>[2x]EFTQLSQSIAEFHTYQLGNGRCSSLLAQRI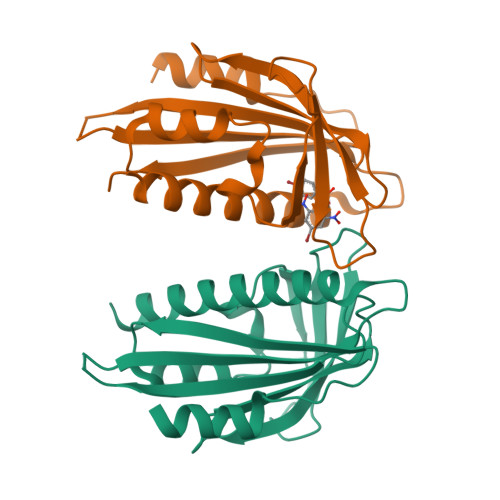HAPPETVWSVVRRFDRPQIYKHFIKSCNVSEDFEMRVGCTRDVNVISGLPANTSRERLDLLDDDRRVTGFSITGGEHRLRNYKSVTTVHRFEKEEEEERIWTVVLESYVVDVPEGNSEEDTRLFADTVIRLNLQKLASITEAMNR(2S)-2-azanyl-3-(4H-1,2,4-triazol-3-yl)propanoic acid | C5 H8 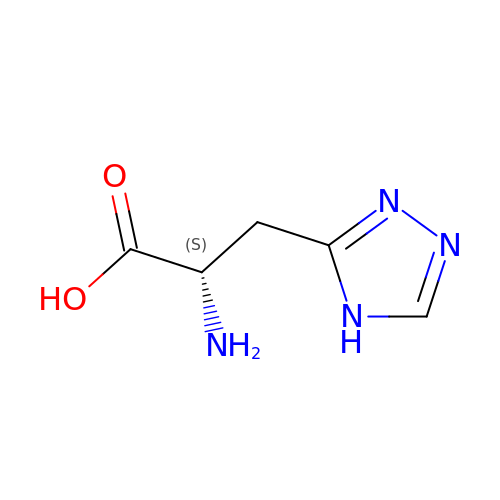N4 O2 | CAPORZWUTKSILW-VKHMYHEASA-N>[2x]SNAMSAVMTPAGFTDYKVADITLAAWGRRELIIAESEMPALMGLRRKYAGQQPLKGAKILGCIHMTIQTGVLIETLVALGAEVRWSSCNIFSTQDQAAAAIAAAGIPVFAWKGETEEEYEWCIEQTILKDGQPWDANMVLDDGGDLTEILHKKYPQMLERIHGITEETTTGVHRLLDMLKNGTLKVPAINVNDSVTKSKNDNKYGCRHSLNDAIKRGTDHLL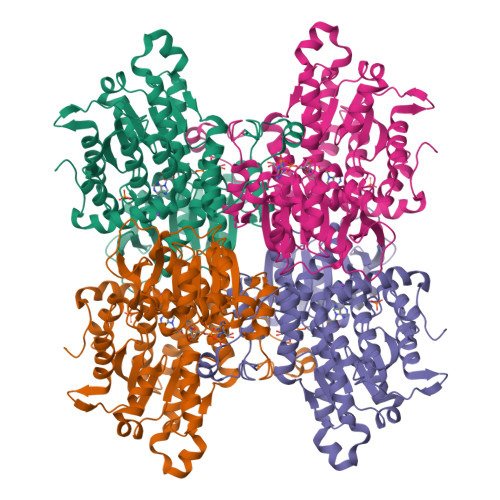SGKQALVIGYGDVGKGSSQSLRQEGMIVKVAEVDPICAMQACMDGFEVVSPYKNGINDGTEASIDAALLGKIDLIVTTTGNVNVCDANMLKALKKRAVVCNIGHFDNEIDTAFMRKNWAWEEVKPQVHKIHRTGKDGFDAHNDDYLILLAEGRLVNLGNATGHPSRIMDGSFANQVLAQIHLFEQKYADLPAAEKAKRLSVEVLPKKLDEEVALEMVKGFGGVVTQLTPKQAEYIGVSVEGPFKPDTYRY>MPSALQGKVALITGASSGIGEATARALAAEGAAVAIAARRVEKLRALGDELTAAGAKVHVLELDVADRQGVDAAVASTVEALGGLDILVNNAGIMLLGPVEDADTTDWTRMIDTNLLGLMYMTRAALPHLLRSKGTVVQMSSIAGRVNVRNAAVYQATKFGVNAFSETLRQEVTERGVRVVVIEPGTTDTE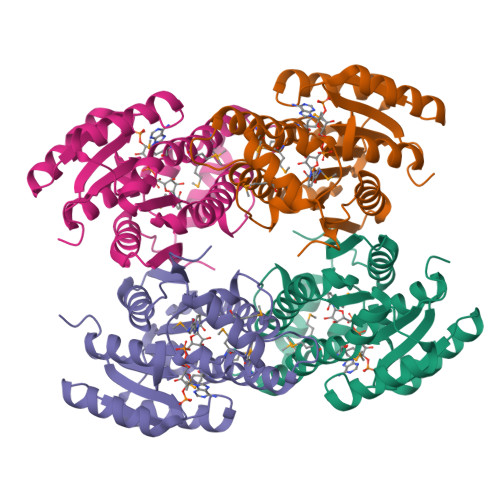LRGHITHTATKEMYEQRISQIRKLQAQDIAEAVRYAVTAPHHATVHEIFIRPTDQV[4x]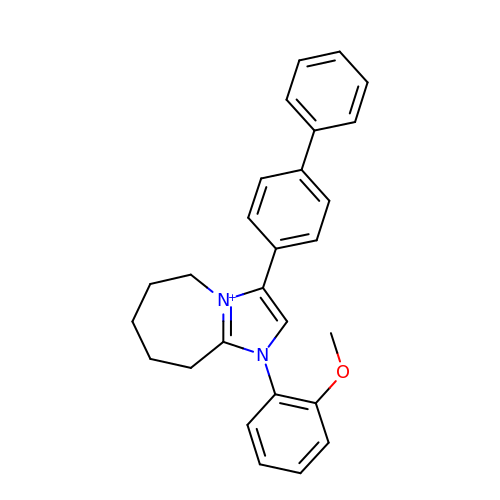8-(2-methoxyphenyl)-10-(4-phenylphenyl)-1$l^{4},8-diazabicyclo[5.3.0]deca-1(7),9-diene | C27 H27 N2 O | ZXQNQLPFZBEUMQ-UHFFFAOYSA-N> VSEIKTLVTFFGGTGDLAKRKLYPSVFNLYKKGYLQKHFAIVGTARQALNDDEFKQLVRDSIKDFTDDQAQAEAFIEHFSYRAHDVTDAASYAVLKEAIEEAADKFDIDGNRIFYMSVAPRFFGTIAKYLKSEGLLADTGYNRLMIEKPFGTSYDTAAELQNDLENAFDDNQLFRINHYLGKEMVQNIAALRFGNPIFDAAWNKDYIKNVQVTLSEVLGVEERAGYYDTAGALLDMIQNHTMQIVGWLAMEKPESFTDKDIRAAKNAAFNALKIYDEAEVNKYFVRAQYGAGDSADFKPYLEELDVPADSKNNTFIAGELQFDLPRWEGVPFYVRSGKRLAAKQTRVDIVFKAGTFNFGSEQEAQEAVLSIIIDPKGAIELKLNAKSVEDAFNTRTIDLGWTVSDEDKKNTPEPYERMIHDTMNGDGSNFADWNGVSIAWKFVDAISAVYTADKAPLETYKSGSMGPEASDKLLAANGDAW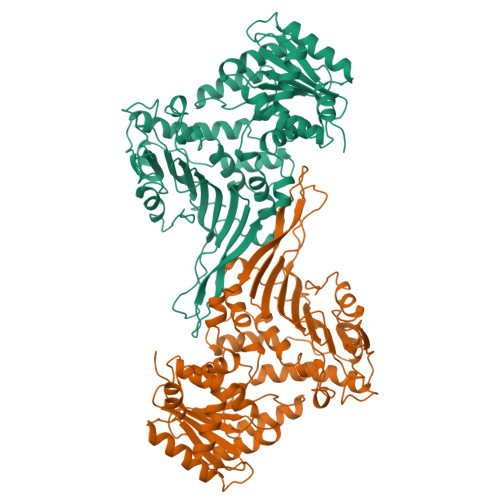VFKG> GEDVFEVEKILDMKTEGGKVLYKVRW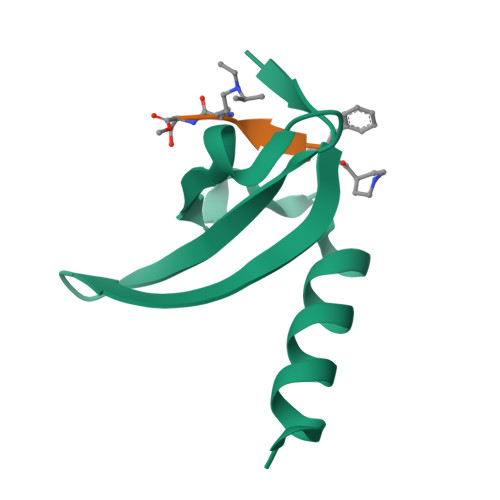KGYTSDDDTWEPEIHLEDCKEVLLEFRKKIAENKAK> MSKLVRSIKNVAGGYSSAQRVVRNATSNDPTGPTTFDMEEISSFTYQSQTEFMEVMDMLDRRLNDKGKNWRHVAKSLTVLDYLV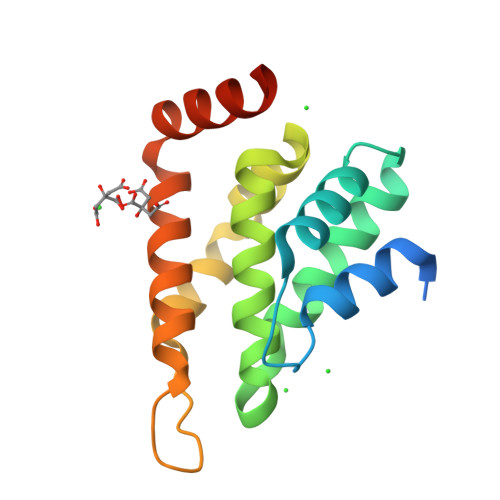RYGSDKCVLWAKDNLYIIKTLREFVHFDETNNDQGAIIRVKAKELVSLLRDDERLKQERANAKKNKRYRSY>[2x]MLGQMMTQPLLISSLIDHAARYHGQTEIVSVETDGTVTRTNWGEIAANARRMGSALTKLGLQPQDRIGTLAWNNRRHLEIYYAASGAGFVCHTINPRLFPEQLVYIINHAQDRVLFFDATFLPLVAAIRDQLTEVKHFVLMGPRNEDALQQIPGLEFYDELIETGDTDFEWPVFDENTASSLCYTSGTTGHPKGVLYSHRSTVLHSFASNTRDVIGYSAMDVVMPVVPMFHVNAWGSPYGCAMSGAQMVLPGPDLHGEALVNLIDTYGVTLAMGVPTIWQGLLAHAAKCGTKLESLERTVIGGAACPPSMIATFREKYGVDTVHAWGMSEMSPLGTANIPLAKHRKLPIEEQHKLRENQGRPPFGVELKIVDDDGNDLPHDGVTQ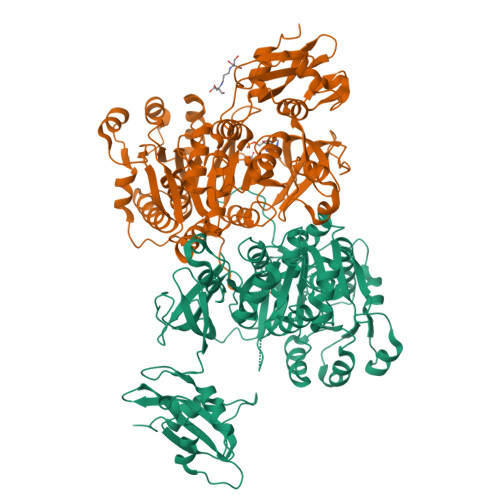GDLMVRGHWVLDSYFQLKDQELLQDGWFATGDVATLDPDGYMTIRDRSKDIIKSGGEWISSVELENIAVAHPKLATAAVIGVPHPKWDERPLLVAVKAEGEDPSEAELLEFFDGKIAKWQVPDKVVFVDALPLNATGAVLKRKLRDEFKDALTG>[2x]SNVPHKSSLPEGIRPGTVLRIRGLVPPNASRFHVNLLCGEEQGSDAALHFNPRLDTSEVVFNSKEQGSWGREERGPGVPFQRGQPFEVLIIASDDGFKAVVGAAQYHHFRHRLPLARVRLV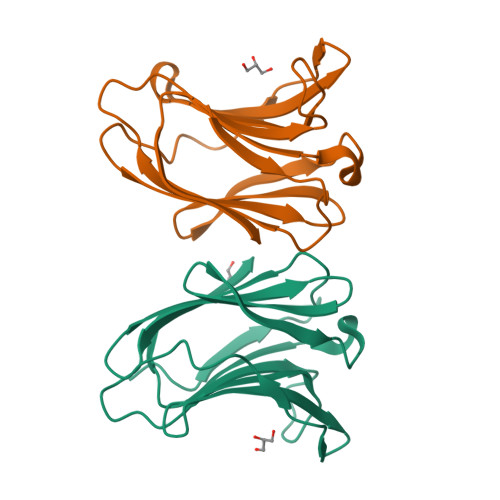EVGGDVQLDSVRIF Among these carbapenemases, OXA-48-like enzymes are widely disseminated and plasmid-encoded, and antibiotic resistance in OXA-48-producing Enterobacterales can lead to high clinical mortality rates. Though the catalytic mechanism of OXA-48 is known, the molecular origin of its biphasic kinetics has been elusive. The partial inactivation of several OXA carbapenemases during turnover has been observed in the literature. It has been proposed that it is a result of the decarbamylation of the N-carbamylated catalytic lysine residue (KCX), which acts as a general base and is critical for the acylation and deacylation steps of the reaction. Our data and analysis thereof show that chloride ion acts as a Janus effector: it delivers allosteric activation by binding at the dimeric enzyme interface while independently causing the inhibition of steady-state catalytic activity by misorientation of a reactive intermediate by ion pairing with R250 in the active site.

To reveal the effect of chloride on imipenem hydrolysis, we sought to obtain a complex structure of OXA-48 in the presence of halides and imipenem. We added 500 mM NaBr and 32 mM imipenem to the apo OXA-48WT crystal and observed a clear Br– anomalous signal overlapping with the density of imipenem, indicating that Br– and imipenem compete for binding to R250 (1.53 Å resolution). R250 has been proposed to play an important role in catalysis by binding to the carboxylate of the substrates. Through mutagenesis and molecular docking, we established that R250 not only is important for substrate binding but also is the target for ion pair-induced enzyme inhibition by chloride. To further explore whether the binding of halides at R250 is a key driving force for the formation of the inactive acyl intermediate, we performed ITC analysis and showed that the OXA-48R250A variant no longer responds to the presence of chloride with biphasic features but the nonconserved OXA-48R214A variant still does. These data indicate that the binding of chloride to R250 is essential for chloride-induced biphasic kinetics. After supplementation of chloride, binding of chloride wedged between the imipenem intermediate and R250 results in progressive rate retardation from the accumulation of the inactive intermediate formed during catalysis until a new active–inactive equilibrium is established to deliver the slower steady-state kinetics observed.

>[4x]MHHHHHHSAGENLYFQGKEWQENKSWNAHFTEHKSQGVVVLWNENKQQGFTNNLKRANQAFLPASTFKIPNSLIALDLGVVKDEHQVFKWDGQTRDIATWNRDHNLITAMKYSVVPVYQEFARQIGEARMSKMLHAFDYGNEDISGNVDSFWLDGGIRISATEQISFLRKLYHNKLHVSERSQRIVKQAMLTEANGDYIIRAKTGYSTRIEPKIGWWVGWVELDDNVWFFAMNMDMPTSDGLGLRQAITKEVLKQEKIIP> MGLFDRIKRVVSSNLNDLVNKAEDPEKMLEQAILEMQEDLVQLRQGVAQAIAAQKRSEKQYNDAQNEINKWQRNAQLALQKGDENLARQALERKKTYTDTSAALKASLDTQSTQVETLKRNLIQLESKISEAKTKKEMLKARITTAKAQEQLQGMVRGMNTSSAMSAFERMEEKVLMQESRAQALGELAGADLETQFAQLEGGSDVDDELAALK

The ESCRT-III-like protein Vipp1 couples filament polymerization with membrane remodeling. It assembles planar sheets as well as 3D rings and helical polymers, all implicated in mitigating plastid-associated membrane stress. PspA activity is triggered by agents that threaten inner membrane integrity, including phage, mislocalized secretins, and antibiotics, whereas Vipp1 is a plastid component in cyanobacteria, algae, and plants, in which it functions in thylakoid membrane biogenesis and repair. Given that two-dimensional (2D) planar sheets share a close geometric relationship with helical lattices, and as a means of understanding the interconnectedness of Vipp1 polymers including rings, spirals and planar sheets, we determined the structure of four Vipp1 helical filaments by cryo-EM.

Specifically, Vipp1 and a Vipp1 interface 3 mutant, Vipp1-F197K/L200K1, were assembled using equivalent helical parameters and lattices and were termed Vipp1L1 and Vipp1F197K/L200K_L1, respectively. Compared with the Vipp1Δα61–219 sample, Vipp1 was characterized by unfurled ring stacks or helical-like ribbons with fewer and shorter ordered helical filaments, suggesting a reduced stability for helical polymerization. Although the Fourier transforms of Vipp1L1 and Vipp1Δα6_L2 class averages were similar with closely related lattices, only helical parameters with a rise of 2.37 Å and a rotation of −75.86° yielded a Vipp1L1 map at an overall resolution of 3.7 Å. Map local resolution range was wider than other Vipp1 helical forms with the inner parts of the filament well resolved compared with the periphery, where the hairpin tips and helix α5 were more poorly ordered. The Vipp1L1 subunit was built between amino acids 1–214 and assembled using similar interfaces as for Vipp1Δα6_L2 and Vipp1Δα6_L3. However, the Vipp1L1 subunit differed from the Vipp1Δα6_L2 and Vipp1Δα6_L3 subunits, with its hairpin tip kinked at Ile68 and helix α5 compacted such that interfaces 1 and 3 were perturbed. Although map relating to the CTD could not be assigned, our structures were consistent with this motif destabilizing interface 1, possibly through kinking of the hairpin while directly or indirectly limiting the formation of interface 3. Compared with Vipp1Δα6_L2 and Vipp1Δα6_L3, the Vipp1L1 filament was constricted with a 21.0 nm and 10.5 nm external and inner diameter, respectively. Specifically, the left-handed 21-start helix in Vipp1Δα6_L2 and Vipp1Δα6_L3 that runs nearly parallel to the helix axis formed a 19-start helix in Vipp1L1. Overall, the comparison of Vipp1L1, Vipp1Δα6_L2, and Vipp1Δα6_L3 filaments provided a mechanism for constriction wherein CTD-mediated adjustments to lattice assembly induced a reduction of ESCRT-III-like protofilaments and consequently a reduction in filament circumference.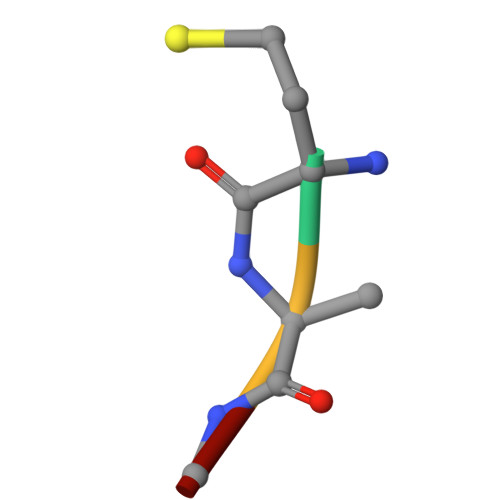> MFLE> MANKRMKVKHDDHYELIVDGRVYYICIVCKRSYVCLTSLRRHFNIHSWEKKYPCRYCEKVFPLAEYRTAHEIHHTGERRYQCLACGKSFINYQFMSSHIKSVHSQDPSGDSKLYRLHPCRSLQIRQYAYLSD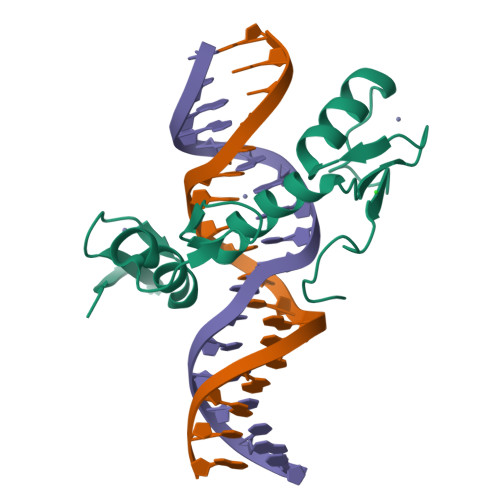RS2-(butanoylamino)thiophene-3-carboxamide 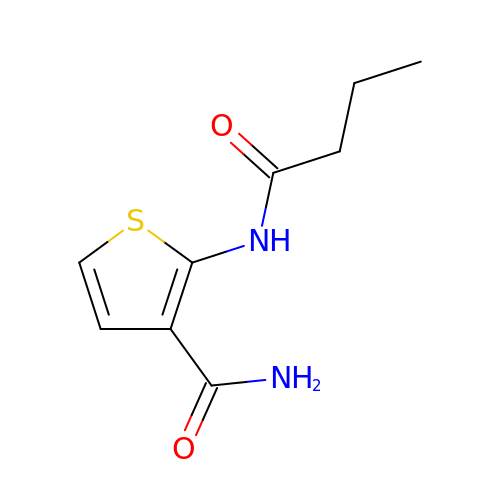| C9 H12 N2 O2 S | QFUOJZBSCYPNSJ-UHFFFAOYSA-N> PHMENEDFCAVCLNGGELLCCDRCPKVFHLSCHVPALTSFPGGEWVCTLCRSLTQPEMEYDSENASHNQPGK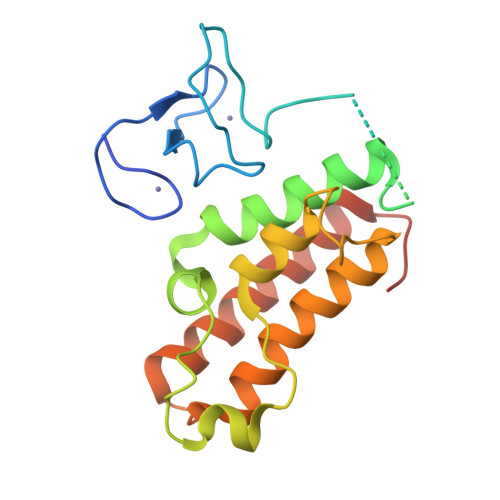RASPGLSMYDQKKCEKLVLSLCCNNLSLPFHEPVSPLARHYYQIIKRPMDLSTIRRKLQKKDPAHYTTPEEVVSDVRLMFWNCAKFNYPDSEVAEAGRSLENFFEGWLKEIYPEKRFAQPRQED>[8x]MLRTMLKSKIHRATVTCADLHYVGSVTIDADLMDAADLLEGEQV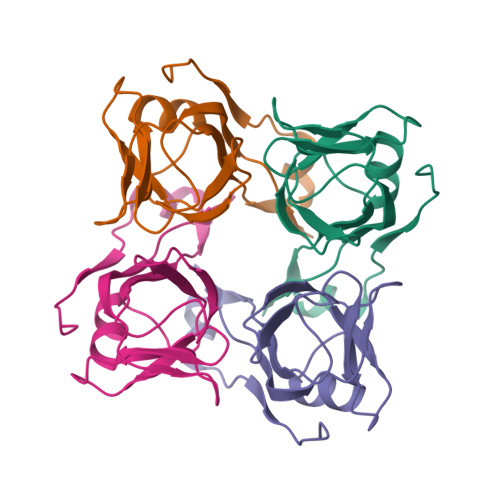TIVDIDNGARLVTYAITGERGSGVIGINGAAAHLVHPGDLVILIAYATMDDARARTYQPRIVFVDAYNKPIDMGHDPAFVPENAGELLDPRLGVG> EKVDNPFEGAKLYVNPVWSAKAAAEPGGSAVANESTAVWLDRIGAIEGNDSPTTGSMGLRDHLEEAVRQSGGDPLTIQVVIYNLPGRACAALAANGELGPDELDRYKSEYIDPIADIMWDFADYENLRIVAIIEIDSL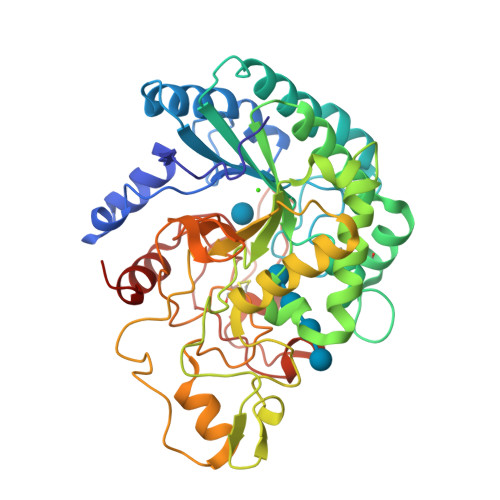PNLVTNVGGNGGTELCAYMKQNGGYVNGVGYALRKLGEIPNVYNYIDAAHHGWIGWDSNFGPSVDIFYEAANASGSTVDYVHGFISNTANYSATVEPYLDVNGTVNGQLIRQSKWVDWNQYVDELSFVQDLRQALIAKGFRSDIGMLIDTSRNGWGGPNRPTGPSSSTDLNTYVDESRIDRRIHPGNWCNQAGAGLGERPTVNPAPGVDAYVWVKPPGESDGASEEIPNDEGKGFDRMCDPTYQGNARNGNNPSGALPNAPISGHWFSAQFRELLANAYPPL>MTLKVILGEHQITRTELLVGIATVSGCGAVVYCISKFWGYGAIAPYPQSGGNRVTRALQRAVIDKTKTPIETRFYPLDSLRTVTPKRVADNGHAVSGAVRDAARRLIDESITAVGGSKFEVNPNPNSSTGLRNHFHFAVGDLAQDFRNDTPADDAFIVGVDVDYYVTEPDVLLEHMRPVVLHTFNPKKVSGFDADSPFTIKNNLVEYKVSGGAAWVHPVWDWCEAGEFIASRVRTSWKEWFLQLPLRMIGLEKVGYHKIHHCRPWTDCPDRALVYTIPQYVIWRFNWIDTELHVRKLKRIEYQDETKPGWNRLEYVTDKNELLVSIGREGEHAQITIEKEKLDMLSGLSATQSVNARLIGMGHKDPQYTSMIVQYYTGKKVVSPISPTVYKPTMPRVHWPVTSDADVPEVSARQYTLPIVSDCMMMPMIKRWETMSESIERRVTFVANDKKPSDRIAKIAETFVKLMNGPFKDLDPLSIEETIERLNKPSQQLQLRAVFEMIGVKPRQLIESFNKNEPGMKSSRIISGFPDILFILKVSRYTLAYSDIVLHAEHNEHWYYPGRNPTEIADGVCE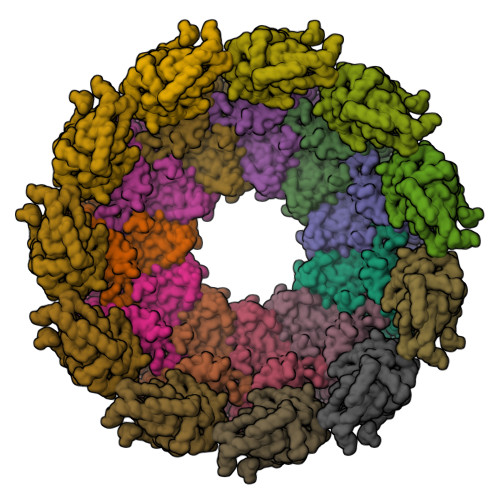FVSDCDAEVIETDFSNLDGRVSSWMQRNIAQKAMVQAFRPEYRDEIISFMDTIINCPAKAKRFGFRYEPGVGVKSGSPTTTPHNTQYNGCVEFTALTFEHPDAEPEDLFRLIGPKCGDDGLSRAIIQKSINRAAKCFGLELKVERYNPEIGLCFLSRVFVDPLATTTTIQDPLRTLRKLHLTTRDPTIPLADAACDRVEGYLCTDALTPLISDYCKMVLRLYGPTASTEQVRNQRRSRNKEKPYWLTCDGSWPQHPQDAHLMKQVLIKRTAIDEDQVDALIGRFAAMKDVWEKITHDSEESAAACTFDEDGVAPNSVDESLPLLNDAKQTRANPGTSRPHSNGGGSSHGNELPRRTEQRAQGPRQPARLPKQGKTNGKSDGNITAGETQRGGIPRGKGPRGGKTNTRRTPPKAGAQPQPSNNRKSRLEEELRRRLTE[22x]> MGSSHHHHHHSSGENLYFQGHMTQQPQAKYRHDYRAPDYQITDIDLTFDLDAQKTVVTAVSQAVRHGASDAPLRLNGEDLKLVSVHINDEPWTAWKEEEGALVISNLPERFTLKIINEISPAANTALEGLYQSGDALCTQCEAEGFRHITYYLDRPDVLARFTTKIIADKIKYPFLLSNGNRVAQGELENGRHWVQWQDPFPKPCYLFALVAGDFDVLRDTFTTRSGREVALELYVDRGNLDRAPWAMTSLKNSMKWDEERFGLEYDLDIYMIVAVDFFNMGAMENKGLNIFNSKYVLARTDTATDKDYLDIERVIGHEYFHNWTGNRVTCRDWFQLSLKEGLTVFRDQEFSSDLGSRAVNRINNVRTMRGLQFAEDASPMAHPIRPDMVIEMNNFYTLTVYEKGAEVIRMIHTLLGEENFQKGMQLYFERHDGSAATCDDFVQAMEDASNVDLSHFRRWYSQSGTPIVTVKDDYNPETEQYTLTISQRTPATPDQAEKQPLHIPFAIEL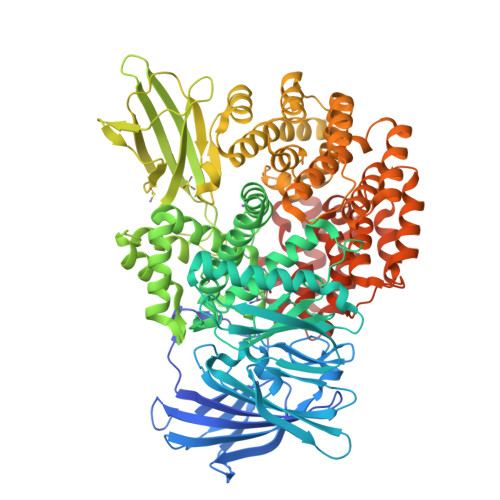YDNEGKVIPLQKGGHPVNSVLNVTQAEQTFVFDNVYFQPVPALLCEFSAPVKLEYKWSDQQLTFLMRHARNDFSRWDAAQSLLATYIKLNVARHQQGQPLSLPVHVADAFRAVLLDEKIDPALAAEILTLPSVNEMAELFDIIDPIAIAEVREALTRTLATELADELLAIYNANYQSEYRVEHEDIAKRTLRNACLRFLAFGETHLADVLVSKQFHEANNMTDALAALSAAVAAQLPCRDALMQEYDDKWHQNGLVMDKWFILQATSPAANVLETVRGLLQHRSFTMSNPNRIRSLIGAFAGSNPAAFHAEDGSGYLFLVEMLTDLNSRNPQVASRLIEPLIRLKRYDAKRQEKMRAALEQLKGLENLSGDLYEKITKALA>MDDQLKQSALDFHEFPVPGKIQVSPTKPLATQRDLALAYSPGVAAPCLEIEKDPLKAYKYTARGNLVAVISNGTAVLGLGNIGALAGKPVMEGKGVLFKKFAGIDVFDIEVDELDPDKFIEVVAALEPTFGGINLEDIKAPECFYIEQKLRERMNIPVFHDDQHGTAIISTAAILNGLRVVEKNISDVRMVVSGAGAAAIACMNLLVALGLQKHNIVVCDSKGVIYQGREPNMAETKAAYAVVDDGKRTLDDVIEGADIFLGCSGPKVLTQEMVKKMARAPMILALANPEPEILPPLAKEVRPDAIICTGRSDYPNQVNNVLCFPFIFRGALDVGATAINEEMKLAAVRAIAELAHAEQSEVVASAYGDQDLSFGPEYIIPKPFDPRLIVKIAPAVAKAAMESGVATRPIADFDVYIDKLTEFVYKTNLFMKPIFSQARKAPKRVVLPEGEEARVLHATQELVTLGLAKPILIGRPNVIEMRIQKLGLQIKAGVDFEIVNNESDPRFKEYWTEYFQIMKRRGVTQEQAQRALISNPTVIGAIMVQRGEADAMICGTVGDYHEHFSVVKNVFGYRDGVHTAGAMNALLLPSGNTFIADTYVNDEPDAEELAEITLMAAETVRRFGIEPRVALLSHSNFGSSDCPSSSKMRQALELVRERAPELMIDGEMHGDAALVEAIRNDRMPDSSLKGSANILVMPNMEAARISYNLLRVSSSEGVTVGPVLMGVAKPVHVLTPIASVRRIVNMVALAVVEAQTQPLHHHHHH[12x]

While reducing NAD(P)+ to NAD(P)H, MEs catalyze the oxidative decarboxylation of the TCA cycle intermediate L-malate to produce the TCA carbon source pyruvate and a byproduct carbon dioxide (CO2) in the presence of divalent metal ions such as a magnesium (Mg2+) ion. The hybrid-type MEs consist of an N-terminal catalytic domain (ME domain) and a C-terminal activity regulating domain. The PTA domain does not possess an enzymatic activity of PTA but acts as an allosteric modulator of catalysis; that is, binding of some metabolites to the PTA domain increases or decreases the enzymatic activity. Binding of acetyl-CoA to the PTA domain is known to reduce the catalytic activity of several hybrid-type MEs.

For structural analysis of EcMaeB, we initially determined the X-ray crystal structure of EcMaeB without cofactors (NADP+ and Mg2+) and the effector ligand acetyl-CoA (EcMaeBapo) at 3.85 Å resolution. There are two almost identical homohexamer of EcMaeB in the asymmetric unit although EcMaeB was previously expected to form a homooctamer based on the results of size exclusion chromatography and native electrophoresis. The EcMaeBapo homohexamer placed the PTA domain and the ME domain on the inside and the outside of the hexameric structure, respectively, as the BbMaeB homohexamer does. The hexamer shows the D3 symmetry, where the 3-fold axis is located at the center of a triangle formed by the PTA domains and 2-fold axes at around the interfaces of four protomers. Here, we define the state represented by this homohexamer as a vertical (V) state because the ME domain dimers are almost vertical to the plane on which 2-fold axes exist. The result that EcMaeBapo is the V state instead of the H state could be due to the effect of molecular packing in a crystal, which can limit possible protein structures. The RMSD calculated using 1900 Cα atoms is 0.51 Å, showing that the PTA domains of EcMaeBholo and EcMaeBapo are almost identical to each other.After a single round of mutagenesis and screening, we obtained a double mutant Cry3Aa–PML I118V, E130G (Cry3Aa–PMLVG) with improved pNPP hydrolysis activity compared to Cry3Aa–PML, resulting in a catalyst with 9% activity retention compared to soluble PML. Previous studies of PML and its homologs have shown that this class of lipases exists in two conformations, an open conformation, and a closed conformation. Current PML structures have only been solved in closed conformations, even when bound covalently to a diethyl phosphonate (DEP) inhibitor.

Nevertheless, crystals of the free PMLVG protein were obtained and its structure was determined by X-ray crystallography to try to gain insight into how the I118V and E130G mutations impact the catalytic efficiency. The overall structure is nearly identical to wild-type PML with the main structural difference being a change in helix α6 near the active site. Helix α6 contains an amino acid hydrophobic patch that has been proposed to be involved in binding to fatty acid substrates. As a consequence of the two mutations, helix α6 changes from an α-helix in PML to a 310 helix in PMLVG that orients its hydrophobic amino acids, particularly I154, into the substrate binding pocket and towards the DEP inhibitor. The net result is a constriction in the size of the substrate-binding channel. The PMLVG channel is large enough to accommodate a fatty acid substrate suggesting that PMLVG should be capable of hydrolyzing pNPP despite being in the closed conformation. Notably, assuming that the closed conformation was active, the tighter binding pocket in PMLVG compared to wild-type PML would be consistent with the lower KM deduced from kinetics. Another structural difference between the PMLVG mutant and wild-type PML is the loop region connecting helices α5 and α6. This loop is visible in the PMLVG structure but absent in wild-type PML suggesting it is more disordered. Soluble PML and PMLVG had T50 values of 45.6 °C and 40.5 °C, respectively, suggesting that the I118V and/or E130G mutations destabilize PML in solution.

> STKYPIVLVHGLAGFNEIVGFPYFYGIADALRQDGHQVFTASLSAFNSNEVRGKQLWQFVQTLLQETQAKKVNFIGHSQGPLACRYVAANYPDSVASVTSINGVNHGSEIADLYRRVMRKDSIPEYIVGKVLNAFGTIISTFSGHRGDPQDAIAALESLTTEQVTEFNNKYPQALPKTPGGEGDEIVNGVHYYCFGSYIQGLIAGEKGNLLDPTHAAMRVLNTFFTEKQNDGLVGRSSMRLGKLIKDDYAQDHIDMVNQVAGLVGYNEDIVAIYTQHAKYLASKQL>[3x]MKGSRIELGDVTPHNIKQLKRLNQVIFPVS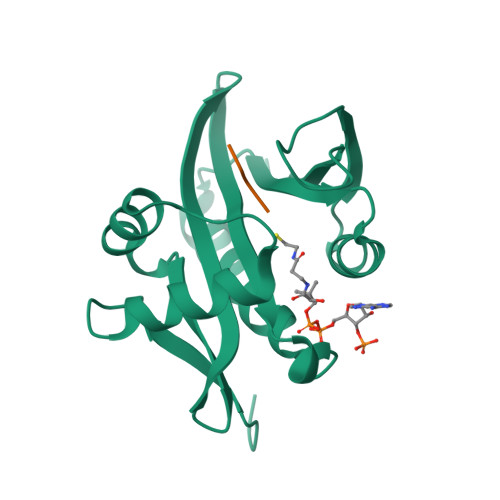YNDKFYKDVLEVGELAKLAYFNDIAVGAVCCRVDHSQNQKRLYIMTLGCLAPYRRLGIGTKMLNHVLNICEKDGTFDNIYLHVQISNESAIDFYRKFGFEIIETKKNYYKRIEPADAHVLQKNLKVPSGQNADVQKTDN;>MLGPEGGRWG[3x]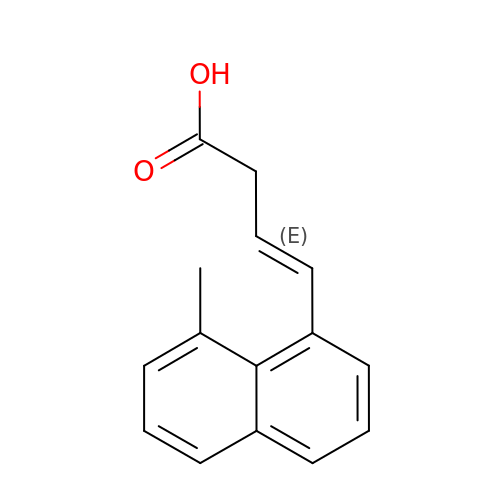(3E)-4-(8-methylnaphthalen-1-yl)but-3-enoic acid | C15 H14 O2 | FALDQPGQWAZNKV-RUDMXATFSA-N>GSELFRGVLQVSSNVLDCANDNWWCSLLDLDTSDWEPLTHTNRLMAIYLSSVASK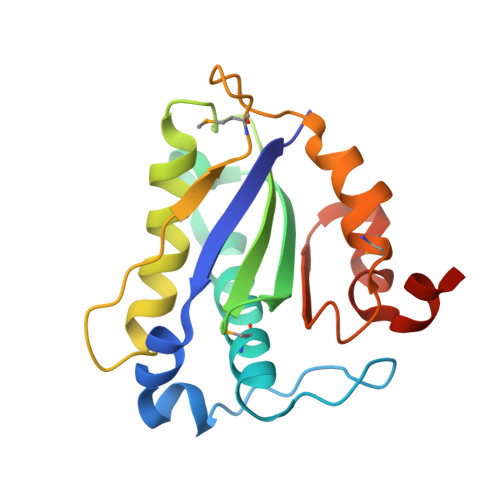LDFTGGPLAGCLYFFQVECNKFEEGYHIHVVIGGPGLNPRNLTVCVEGLFNNVLYHLVTGNVKLKFLPGMTTKGKYFRDGEQFIENYLMKKIPLNVVWCVTNIDGYIDTCISATFRRGACHA[2x]>[3x]GPLGSMVDYIVEYDYDAVHDDELTIRVGEIIRNVKKLQEEGWLE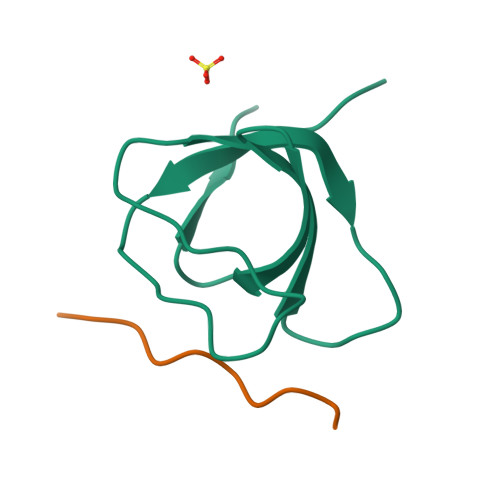GELNGRRGMFPDNFVKEIKRE;>AKKNLPTAPPRRRVSE[3x]>[2x]SKSDVFHLGLTKNDLQGAQLAIVPGDPERVEKIAALMDKPVKLASHREFTSWRAELDGKAVIVCSTGIGGPSTSIAVEELAQLGIRTFLRIGTTGAIQPHINVGDVLVTTASVRLDGASLHFAPMEFPAVADFACTTALVEAAK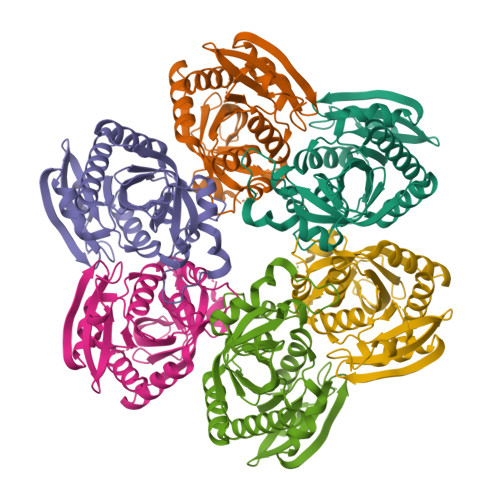SIGATTHVGVTASSDTFYPGQERYDTYSGRVVRRFKGSMEEWQAMGVMNYEMESATLLTMCASQGLRAGMVAGVIVNRTQQEIPNAETMKQTESHAVKIVVEAARRLL>[2x]ECHLSDLLQQLTSVNASKPSERGLVRQEEAEDPACIPIFWVSKWVDYSDKYGLGYQLCDNSVGV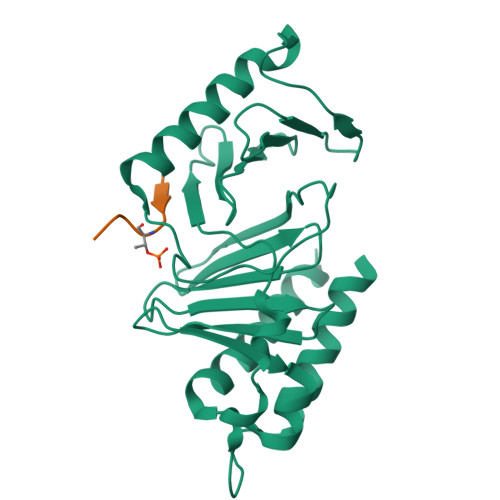LFNDSTRLILYNDGDSLQYIERDGTESYLTVSSHPNSLMKKITLLNYFRNYMSEHLLKAGANITPREGDELARLPYLRTWFRTRSAIILHLSNGTVQINFFQDHTKLILCPLMAAVTYINEKRDFQTYRLSLLEEYGCCKELASRLRYARTMVDKLLSSR;>[2x]LHYPSTTALQE> STNMLEALQQRLEKYQSVEAAAKAENNSGKARRFGRIVKQYEDAIKLYKAG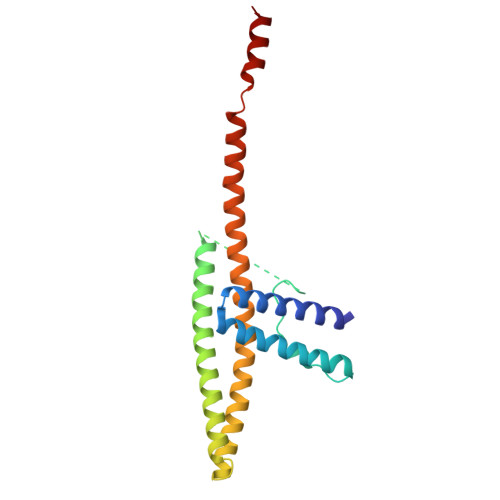KPVPYDELPVPPGFGGGGGGGGGGGTTGEAIQKLRETENMLIKKQEFLEAKIEDELNIARKNASKNKEVALQALKKKKELEKQLQQIDGTLSTIEMQREALESANTNTAVLTTMKNAADALKRAHQNMDVDKVHDMMDD>[2x]GPGSMSNSYEGCGDLTIFVAVALNKVIGHKNQIPWPHITHDFRFLRNGTTYIPPEVLSKNPDIQNVVIFGRKTYESIPKASLPLKNRINVILSRTVKEVPGCLVYEDLSTAIRDLRANVPHNKIFILGGSFLYKEVLDNGLCDKIYLTRLNKEYPGDTYFPDIPDTFEITAISPTFSTDFVSYDFVIYERKDCKTVFPDPPFDQLLMTGTDISVPKPKYVACPGVRIRNHEEFQYLDILADVLSHGVLKPNRTGTDAYSKFGYQMRFDLSRSFPLLTTKKVALRSIIEELLWFIKGSTNGNDLLAKNVRIWELNGRRDFLDKNGFTDREEHDLGPIYGFQWRHFGAEYLDMHADYTGKGIDQLAEIINRIKTNPNDRRLIVCSWNVSDLKKMALPPCHCFFQFYVSDNKLSCMMHQRSCDLGLGVPFNIASYSILTAMVAQVCGLGLGEFVHNLADAHIYVDHVDAVTTQIA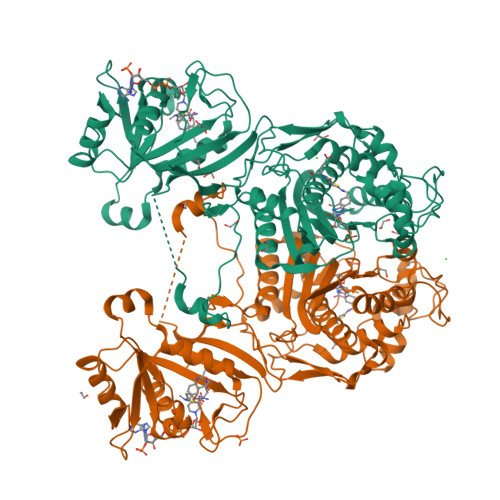RIPHPFPRLRLNPDIRNIEDFTIDDIVVEDYVSHPPIPMAMSA> HGYVSSIQANGQTYPGADPHNPNPESPGWQAENTDLGFVEPSAFSTPAIACHKNARAPPAHATVQAGSTIKLTWNTWPESHHGPVLDYIAPCNGDCSSASAGSLNFVKIAEKGLISGSNPGFWAADELIQNGNSWEVTIPANLAPGKYVLRHEIIALHSAGNPNGAQAYPQCINLEVTGGGSATPSGQPATSFYSPNDPGILFNLYQSFDSYPIPGPAVWSG

Discovered a little over a decade ago, LPMOs are metalloenzymes that utilize a copper ion to catalyze the oxidative cleavage of oligosaccharides and polysaccharides. The thermophilic fungus Malbranchea cinnamomea contains a host of enzymes that enable its ability as an efficient degrader of plant biomass and that could be mined for industrial applications. This thermophilic fungus has been studied and found to encode eight lytic polysaccharide monooxygenases (LPMOs) from auxiliary activity family 9 (AA9), which collectively possess different substrate specificities for a range of plant cell-wall-related polysaccharides and oligosaccharides. Most significantly, McAA9F has a broad substrate specificity, with activity on both crystalline and soluble polysaccharides. The structure of McAA9F represents the first structurally determined AA9 LPMO from M. cinnamomea.

The protein crystals grew as needle clusters; a data set was collected to 1.38 Å resolution and the structure was solved by molecular replacement. A fluorescence scan revealed the presence of a copper ion in the crystallized protein, which as expected was found to be co­ordinated by the hydroxyl of Tyr169 and the histidine brace: Nδ of His1 and Nɛ2 of His81. A succinimide is observed in place of Asp10, which is found in a turn connecting β1 and β2. McAA9F is the first reported AA9 to contain a succinimide modification. In comparison to TaAA9A, the L2 region in McAA9F is shorter by five residues and lacks the helical motif. McAA9F also lacks the conserved tyrosine residue of the motif, but instead possesses a histidine residue (His20), the imidazole side chain of which occupies an equivalent position and is likely to fulfill an equivalent proposed substrate-stacking role. Interestingly, McAA9F showed activity on both crystalline cellulose and on soluble substrates while containing an extremely short L3 loop aligned to the surface level, indicating that the absence of an extended L3 is not sufficient to define a lack of activity towards soluble substrates and oligosaccharides. While L3 in McAA9F contains hydrophilic residues capable of interacting with substrates, its considerably smaller size results in the loop being set back >5.5 Å from the +2 sites observed in CvAA9A and LsAA9A. In the crystal form of McAA9F that we obtained, the putative substrate-binding surface is heavily hindered by crystal contacts and thus it would not be possible to pursue ligand complexes using this crystal form.>MATRPTSVEMEPIDDSHHLDKILLQARELSQPIIIDWMASWCGPCIYLKPKLEKLAAEYDTKIKFYCADVNKVPQALVKRGNISKMPTIQLWKDGEMK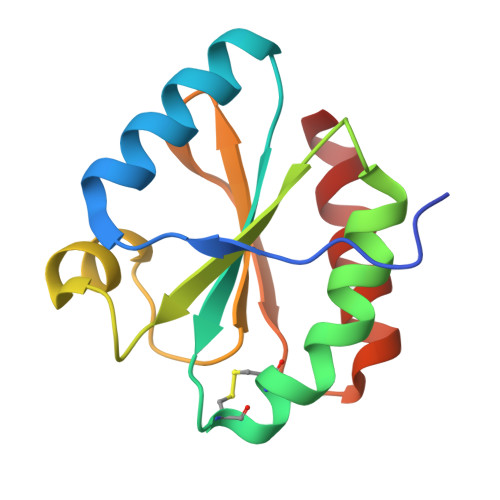AEVIGGHKAWLVIEEVREMIQKFV[2x]2-aminobenzene-1,4-dicarboxylic acid | C8 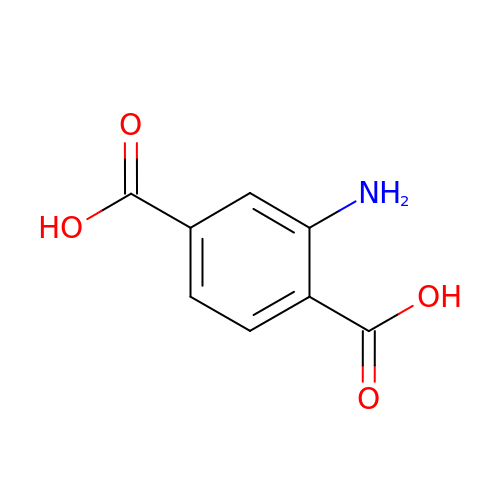H7 N O4 | GPNNOCMCNFXRAO-UHFFFAOYSA-N6-bromo-2-(1-methyl-1H-imidazol-5-yl)-7-{4-[(5-methyl-1,2-oxazol-3-yl)methyl]piperazin-1-yl}-1H-imidazo[4,5-b]pyridine 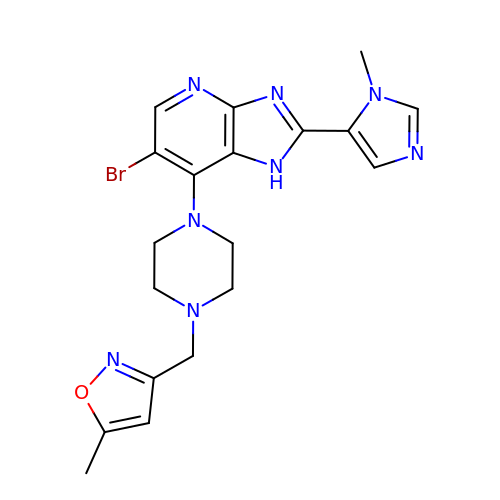| C19 H21 Br N8 O | QWRJMSZUKHRINI-UHFFFAOYSA-N Glycoside phosphorylases (GPs) are carbohydrate-active enzymes that catalyze the reversible cleavage of glycosidic bonds using inorganic phosphate. One of the most well-studied GPs in that regard is sucrose phosphorylase (SP; EC 2.4.1.7), which catalyzes the phosphorolysis of sucrose into α-d-glucose 1-phosphate (Glc1P) and d-fructose. Instead, a clear preference for sucrose 6F-phosphate was observed, making it the first sucrose 6F-phosphate phosphorylase (SPP; EC 2.4.1.329) ever reported. Crystal structures of the two SPPs were determined to allow for a comparison of their active site.

Furthermore, the T. thermosaccharolyticum SPP (TtSPP) was shown to accept an even wider range of substrates than the known SPs, offering opportunities for biotechnological applications and further engineering. The IcSPP crystals contained one protein molecule in the asymmetric unit, whereas the TtSPP crystals contained two. IcSPP seems to exist as a monomer, whereas TtSPP in the crystal structure forms dimers. Thus, the dimers observed in the TtSPP crystals probably do not represent a functional state of the protein. Residues that form hydrogen bonds to the glucosyl group are highly conserved, both in sequence and in structure (Asp49, His87, Arg195, His295, Arg399 in TtSPP). The same is evidently true for the catalytic nucleophile and general acid/base at the tips of β-sheets 4 and 5 of the (β/α)8-barrel, and the aspartate that crucially stabilizes the transition state. These catalytic residues are, respectively, found at Asp197, Glu238, and Asp296 in TtSPP. One tetrahedral sulfate ion is present in subsite +1 of TtSPP. It is held by hydrogen bonds with Tyr201, Arg134, and His344. Arg134, Arg195, Tyr201, His344, Gln345, and Arg399 fulfill this role in TtSPP. In TtSPP, on the other hand, a histidine residue is present instead.

>MGGSHHHHHHGMASMALKNKVQLITYPDSLGGNLKTLNDVLEKYFSDVFGGVHILPPFPSSGDRGFAPITYSEIEPKFGTWYDIKKMAENFDILLDLMVNHVSRRSIYFQDFLKKGRKSEYADMFITLDKLWKDGKPVKGDIEKMFLRRTLPYSTFKIEETGEEEKVWTTFGKTDPSEQIDLDVNSHLVREFLLEVFKTFSNFGVKIVRLDAVGYVIKKIGTSCFFVEPEIYEFLDWAKGQAASYGIELLLEVHSQFEVQYKLAERGFLIYDFILPFTVLYTLINKSNEMLYHYLKNRPINQFTMLDCHDGIPVKPDLDGLIDTKKAKEVVDICVQRGANLSLIYGDKYKSEDGFDVHQINCTYYSALNCDDDAYLAARAIQFFTPGIPQVYYVGLLAGVNDFEAVKKTKEGREINRHNYGLKEIEESVQKNVVQRLLKLIRFRNEYEAFNGEFFIEDCRKDEIRLTWKKDDKRCSLFIDLKTYKTTIDYINENGEEVKYLV[2x]> MHHHHHHTIVDETLNGNPEDTAHSSLSTAAARNLATTTKTVPQMQGITSRWLLRLLPWVQVSGGTYRVNRRLSHTVGDGRIDFDISGSDVAIIPEELRELPALRDFTDTEVLAALGERFTQREYAPGELIAEAGRPGDRLVLIAHGRVDRIGTGKYGDTTVLAALAGGDHLGDAPLTSDEVTWEFSYRAVTRVTVVELPRRAALEIIERSPGLREHLAGVRQGPVHPTNSSGESAVAVASGHRGEPSLPGAFADYDLAPREYELSVAQTVLRT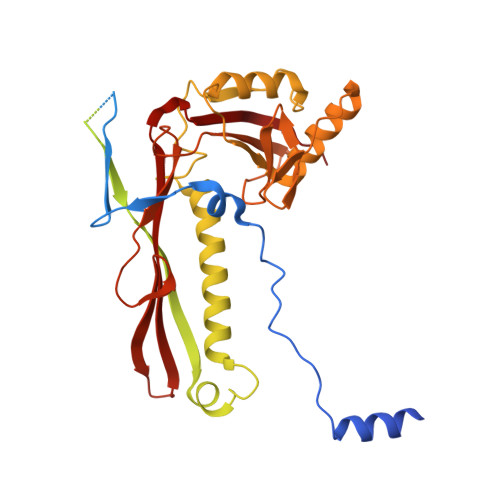HTRVGDLYNDPMNQVEEQLKLTVQALRERQEHEMINNREFGLLHNADLKQRIPTRSGPPTPDDLDDLLATVWKDPGFLLAHPRAIAAMAREWSARGLYPTAVDFHGHSLPSWRGVPIFPCNKIPVTKERTSSILLLRTGEEKQGVVGLHQTGIPDEYEPSLSVRFMGIDDRAVINYLVSAYYSAAVLVPDALGVLEDVEVGL> GSHMNQCPEHSQLTTLGVDGKEFPEVHLGQWYFIAGAAPTKEELATFDPVD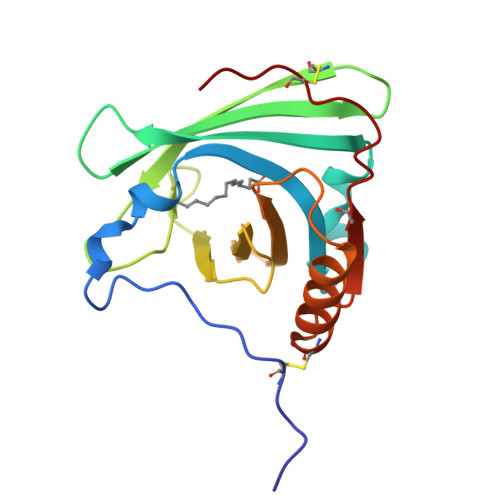NIVFNMAAGSAPMQLHLRATIRMKDGLCVPRKWIYHLTEGSTDLRTEGRPDMKTELFSSSCPGGIMLNETGQGYQRFLLYNRSPHPPEKCVEEFKSLTSCLDSKAFLLTPRNQEACELSNN> PSPSSFPHYSRRHFKRQSPRQLHQLASNLAARGCTDVVLWSSMIQRAIEVNRSPESGAADVSVAPFRFFEALGFLGAVSSLGLTDRELFLSFVPCFLRSLSALEPRHLVQLLTVYEAAGVRPRGLYVAVFNRVLKLAPSFYSHEFADFLCCLARLKIANPSFLSAFSQTLVSRLPEIAF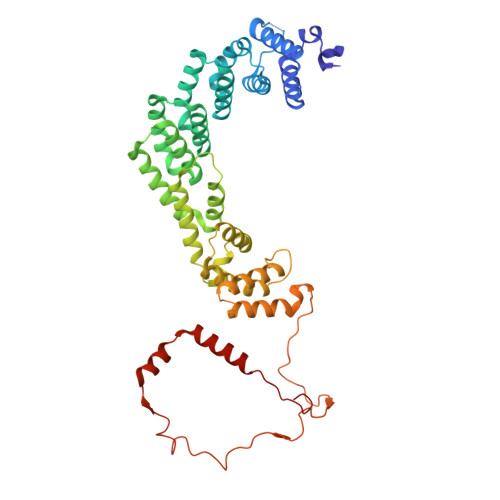PDACRCVGALRSLGVAQQSLFDLFDERQKKELELLPTQLLLEDFQKVLSLEFSWQAYENMIQEEFIKRTEAMIDDKDVDELADPFACLNFMKTRNLVSDKFLLALSKWCRAAVNRPATRSYKRPLAHQLVELHDLMRERNLEQNKALEQAVLRFVADDGGCKRRPREVKPLLYQRNRRYISCPDLIPDGIEPARPCAEALPDVFMERQASLVRACTPEDLARQELPFAVQAETAYRRLQRNKRFLRFVQEE3-[1-(phenylmethyl)indol-6-yl]-1~{H}-pyrazol-5-amine 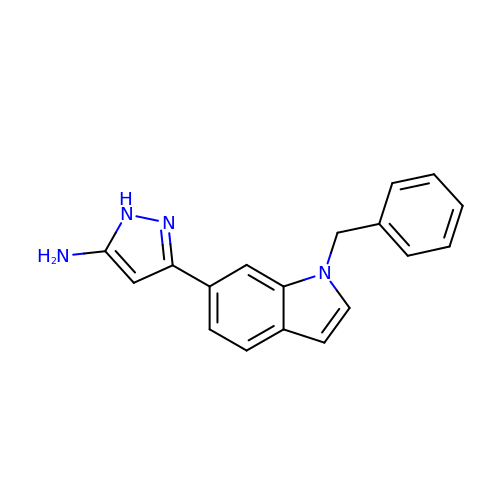| C18 H16 N4 | IXGUTMYAJBKSPV-UHFFFAOYSA-N> MKIANEFTVSVPIEDAWDLLTDLDQVVPLMPGARLTGHDGDDVLGAVKVKVGPVTSEFAGKVHFVEQDREHFRAVIDAKGKETRGTGNAAATVTAQLHEAGT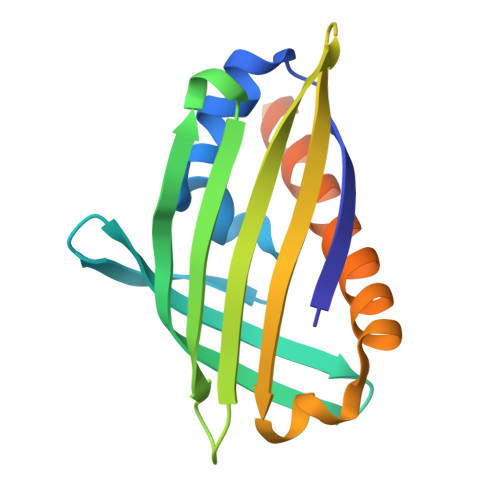STRVTVDTDLKVVGKLAQFGSGMLQQVSEKLLGQFVDSLEAKLAGEREKPSETTQGSLEHHHHHH> PISPIETVPVKLKPGMDGPKVKQWPLTEEKIKALVEICTEMEKEGKISKIGPENPYNTPVFAIKKKDSTKWRKLVDFRELNKRTQDFWEVQLGIPHPAGLKKKKSVTVLDVGDAYFSVPLDEDFRKYTAFTIPSINNETPGIRYQYNVLPQGWKGSPAIFQSSMTKILEPFKKQNPDIVIYQYMDDLYVGSDLEIGQHRTKIEELRQHLLRWGLTTPDKKHQKEPPFLWMGYELHPDKWTVQPIVLPEKDSWTVNDIQKLVGKLNWASQIYPGIKVRQLCKLLRGTKALTEVIPLTEEAELELAENREILKEPVHGVYYDPSKDLIAEIQKQGQGQWTYQIYQEPFKNLKTGKYARMRGAHTNDVKQLTEAVQKITTESIVIWGKTPKFKLPIQKETWETWWTEYWQATWIPEWEFVNTPPLVKLWYQLEK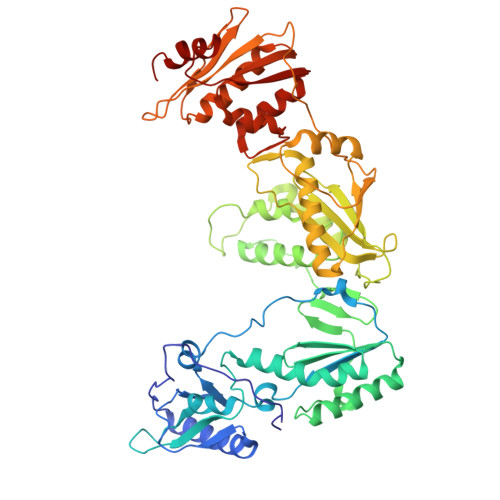EPIVGAETFYVDGAANRETKLGKAGYVTNKGRQKVVPLTNTTNQKTELQAIYLALQDSGLEVNIVTDSQYALGIIQAQPDKSESELVNQIIEQLIKKEKVYLAWVPAHKGIGGNEQVDKLVSAGIR> ENGYTYEDYKNTAEWLLSHTKHRPQVAIICGSGLGGLTDKLTQAQIFDYSEIPNFPRSTVPGHAGRLVFGFLNGRACVMMQGRFHMYEGYPLWKVTFPVRVFHLLGVDTLVVTNAAGGLNPKFEVGDIMLIRDHINLPGFSGQNPLRGPNDERFGDRFPAMSDAYDRTMRQRALSTWKQM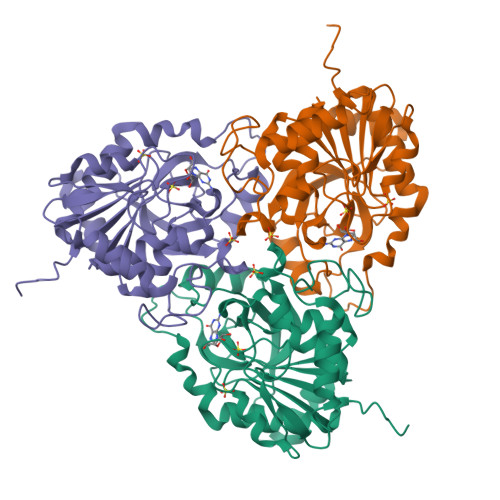GEQRELQEGTYVMVAGPSFETVAECRVLQKLGADAVGMSTVPEVIVARHCGLRVFGFSLITNKVIMDYESLEKANHEEVLAAGKQAAQKLEQFVSILMASIPLPDKAS>[4x]GGGGSMSTAEPAPDPTNPSTSGLAPTTNGIGSPPPTASAATKFSILTKFLRRKNQVHTTTAQQNEFMQKYMPNGNSNAVQPAATGGQPASSDGGSAIEVPPPKESYAVRIRKYLANYTQDPSTDNFYYWTCVVTVAYIYNLLFVIARQVFNDLIGPSSQSLCRFYNGTLNSTTQVECTYNMLTNMKEMPTYSQYPDLGWSKYWHFRMLWVFFDLLMDCVYLIDTFLNYRMGYMDQGLVVREAEKVTKAYWQSKQYRIDGISLIPLDYILGWPIPYINWRGLPILRLNRLIRYKRVRNCLERTETRSSMPNAFRVVVVVWYIVIIIHWNACLYFWISEWIGLGTDAWVYGHLNKQSLPDDITDTLLRRYVYSFYWSTLILTTIGEVPSPVRNIEYAFVTLDLMCGVLIFATIVGNVGSMISNMSAAWTEFQNKMDGIKQYMELRKVSKQLEIRVIKWFDY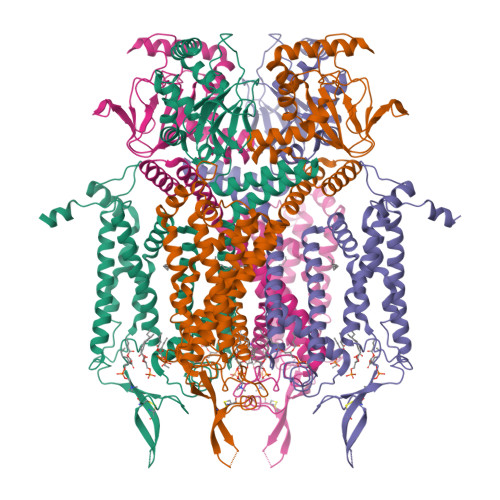LWTNKQSLSDQQVLKVLPDKLQAEIAMQVHFETLRKVRIFQDCEAGLLAELVLKLQLQVFSPGDFICKKGDIGREMYIVKRGRLQVVDDDGKKVFVTLQEGSVFGELSILNIAGSKNGNRRTANVRSVGYTDLFVLSKTDLWNALREYPDARKLLLAKGREILKKDNLLDENAPEEQKTVEEIAEHLNNAVKVLQTRMARLIVEHSSTEGKLMKRIEMLEKHLSRYKALARRQKTMHGVSIDGGDISTDGVDERVRPPRLRQTKTIDLPTGTESESLLK>[4x]G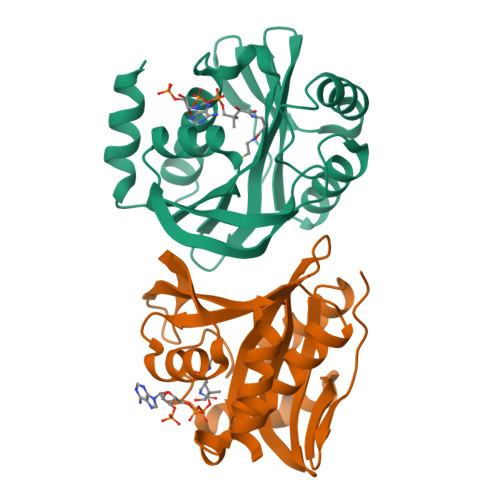HMSRRAPMFKPLPITLQRGALRLEPLVEADIPELVSLAEANREALQYMDGPTRPDWYRQSLAEQREGRALPLAVRLGVQLVGTTRFAEFLPALPACEIGWTWLDQAQHGSGLNRMIKYLMLKHAFDNLRMVRVQLSTAASNLRAQGAIDKLGAQREGVLRNHRRLAGGRLDDTFVYSITDHEWPQVKAALEASFTG In the other class of self-sufficient P450s, CYP116 P450s contain an N-terminal heme domain fused to a phthalate dioxygenase-type reductase domain that consists of a NAD(P)H reductase domain and a [2Fe-2S] cluster-containing domain (ferredoxin) at the C-terminus. The electron transport chain of these P450s is NAD(P)H→FMN→[2Fe-2S]→heme. Notably, CYP116B46 from T. thermophilus is a highly potent and thermostable protein. A more recent report describes its activity in catalyzing region- and enatio-selective C-H-lactonizations of saturated fatty acids.

The heme domain is very similar to the recently reported N-terminal region of CYP116B46 (denoted CYP116B46-N), albeit a small structural difference is observed with Cα root-mean-square deviation, Cα RMSD, of 1.154 Å27. In particular, helix αB’, αE, αF, and αG in CYP116B5-N and CYP116B46-N adopt various conformations.

> QSSVGGCPVHRLAEDFDPFQDAYMADPAQFVRWAREQVPIFYAPKLNYWVVTRYDTIKQIFRDPVTFSPSNVLQSFAQPSAEVRQVLERYGYAFNRTLVNEDEPMHLERRRVLMEPFASEHLAEHEPMVRELVRRAVNRFIDTGRADLVDQMIWEVPFTVALHFLGVDDDDREKMRRFAIAHTVNAFGRPSPEEQLAVAETVGQFWQFCGEVLEKMRRTADGPGWMRYSIRQQKLYPDVVTDSYLHSMMQAIIVAAHETTVFATTNALKTLLEHETVWREICADPSLIPAAAEECLRYNGPVAGWRRRTTREVEVEGVRLPVGANILMVVASANHDSAHFDDPEFFDIGRSNASEHLNFGYGAHQCLGRNLGRMEMQIMIEELSRRLPHMRLAEQRFDYLHNVSFRAPRHLWVEWDPAQNPERRDP>REKGIVEPSCGVTANAIMKLFLDKDGFSYCFENEQTLSLEQLQERLSCMPECKSFVLRVNDGALGHAYIVDIPKGENSCRPAFLYQSDLGEGVTRKLRFEDWMTHKALTPILLDDICNYFSCMSQNKTDLEQIATLFDIDGNVKMLRKENIQYQKHDNFSFQLFEYDTDNIEKN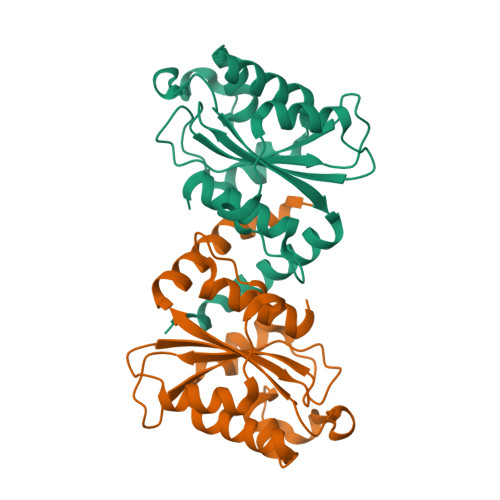IEIIKSLCSGAAALEHHHHHH[2x]> PIFLNVLEAIEPGVVCAGHDNNQPDSFAALLSSLNELGERQLVHVVKWAKALPGFRNLHVDDQMAVIQYSWMGLMVFAMGWRSLTNVNSRMLYFAPDLVFNEYRMHKSRMYSQCVRMRHLSQEFGWLQITPQEFLCMKALLLFSIIPVDGLKNQKFFDELRMNYIKELDRIIACKRKNPTSCSRRFYQLTKLLDSVQPIARELHQFTFDLLIKSHMVSVDFPEMMAEIISVQVP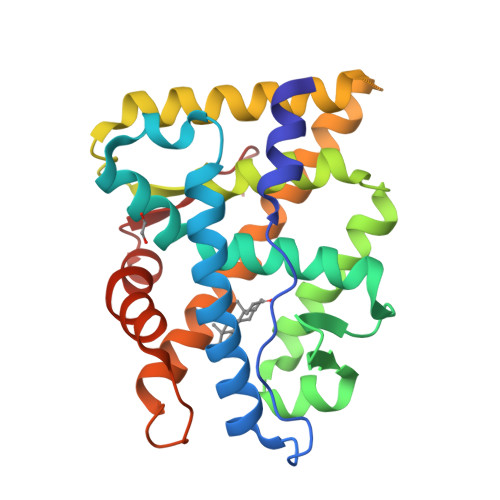KILSGKVKPIYFHTQ> MAVEGKKFDGREAKKGLFFSPHAWGWITHGMFLLLLLPMPLFFCSLWTHLRECCCCPSGPLRLSSGHVERHAKGIVQQMRRTLRHGYHAYVPKGALLKTDMLASSPQLVTAVFRETEAAAERADRANDYAGFFSRPRLNYPVASGIPAFISRRQFDVQYNIFHHDAVATLNRHTLGTSLEGHSLETVIRRASFDATQAAVHTAAAEHFNYCFFYKSLRPWGTAVPKQLREAFQLQYGRDGSVDVVEEVKRLFTVVV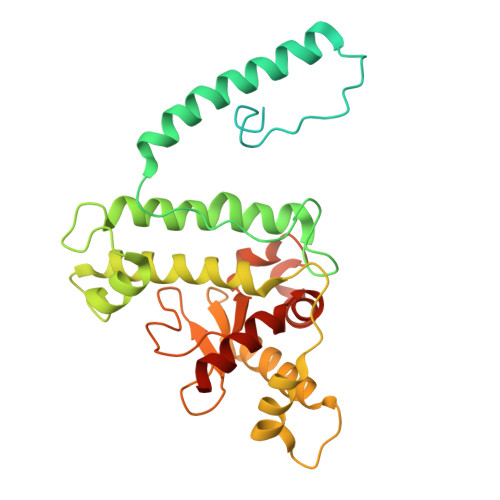LSHQERCGWVYLVWTGKQFDVVEFPHGACPIGSDLIPLLAINVHEGAYSLDYGPSGLEQYAQNYFRACNWFLAERYYLQATGRGSSCDA>[3x]METKMTSFYKITAYNSQALYFWGTDADVDRYVDWL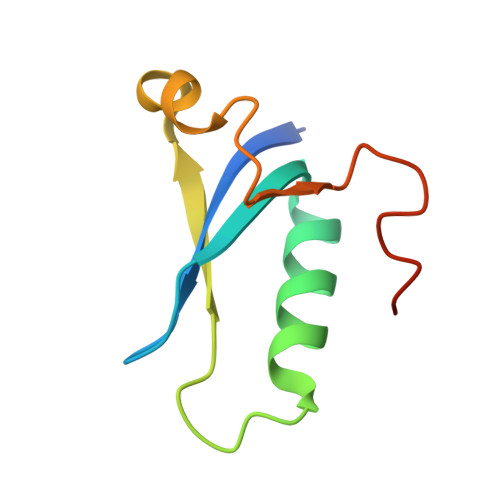NRDREINVYAAEAIPEAEWAQYEGRDDVLSGEECGWDDFMSAEA> MEIVYKPLDIRNEEQFASIKKLIDADLSEPYSIYVYRYFLNQWPELTYIAVDNKSGTPNIPIGCIVCKMDPHRNVRLRGYIGMLAVESTYRGHGIAKKLVEIAIDKMQREHCDEIMLETEVENSAALNLYEGMGFIRMKRMFRYYLNEGDAFKLILPLT;> GPMEVDSILGSLSITDDFDQLVDVTSLFDELCSKLKPEAIVKDPRFDLFEGTHSLEVNNSKLDSSLIELTAEEIEFDVNVAYDPPLASVAAIADRLLRCVISWLNDYQTLPTTVLSCRYTESLLSSLVKGTTAGSSWCTGNILYDKVLGSCILGVCYLTKFVQKLLSAGIVFEEEDLNFNNMGFNTFDNLPGQDVVINSLTESLQILEAYSDDSLHLTMLKHILKIIICLVHLEDHLTDYSTKTSHLDELIENANSVNGIFPQLQLSPPKGAFSTYIQKHRSNQFPPRKITKLPTDYSGFITLANDVKTILLVDKAESALETYQFAKFFNKLEQRHVIARILFPLFFIRDDRTVLGKFSYTQFYLLHVKEFSAQTPSEFESSIGNELIQESSNMLLEWYQNCSQNTCRYRQGFNRQLILWDSLQAQFESVNSQVYCSWTYFMKLSSMIEFSLKGFDLDIYKPFEAYSMFWYVYYLSHHLETFLKDSQNDIESNINAIHSMNKKLKKLKAGEKKDQLRLKYRFAMDNEMEQLQATKQFLNYLLKEINITKSLCLIEVFQFAILKSFGLIDNKNSTPSKFSNERLIHNLRFKPFNSIGVPELPEYEVFQQTLKDFVIEEKGAAFDIKLERATNFIETEVRNVVSSIDEIMQGIKGGDNNGVLVTGTRLVQELSLEYYCKLKHTSKALSVNSKVIVNTLKKNIKNKDSHEYKVELVHTTEGWNYFPIQTLRIKQDRYK;> MDILKLSDFIGNTLIVSLTEDRILVGSLVAVDAQMNLLLDHVEERMGSSSRMMGLVSVPRRSVKTIMIDKPVLQELT;> MLRFVGSRRR

The transfer of an acetyl group from acetyl-coenzyme A to the free α-amino group on the N-terminus of substrate proteins is catalyzed by N-terminal acetyltransferases (NATs), and is considered to be irreversible, as no Nt-deacetylase has been identified so far. NatC acetylates protein N-termini starting with methionine, followed by a hydrophobic or amphipathic amino acid, with amino acids at positions 3 and 4 also contributing to NatC recognition. NatC forms a heterotrimeric complex, containing the catalytic subunit Naa30, the small auxiliary subunit Naa38 and the large auxiliary subunit Naa35. The large auxiliary subunit Naa35 acts as the central assembly hub of the NatC complex, forming extensive interactions with Naa30 and Naa38.

To obtain insights into the substrate recognition mode and the marked difference of NatC catalytic efficiencies toward the two peptides, crystal structures of NatC in complex with CoA, and either yArl3 or Gag peptide were determined to a maximal resolution of 2.99 and 2.75 Å, respectively. The electron density of the peptide ligands was sufficient to model the first four and six amino acids of the yArl3 and Gag peptide, respectively. At peptide position 3, Gag-Arg3 forms a hydrogen bond with the protein backbone and a cation–π interaction with Naa30-Tyr144. In addition, Naa30-Glu29 interacts with the Gag peptide backbone. Only in the Gag peptide, the fourth peptide residue, Phe4, deeply inserts into a second hydrophobic surface generated by Naa30 and Naa35, the “extended pocket”. In particular, binding of the Gag peptide induced a marked constriction of the central tunnel in NatC. Binding of Gag induces a flipping of Leu27, allowing recognition of the N-terminal methionine, which is sandwiched between Leu27 and Tyr145 of Naa30. In contrast to the yArl3 peptide, binding of the viral Gag peptide induced a large conformational rearrangement of the β6–β7 loop in Naa30. Naa30-Asn147 forms a hydrogen bond with Naa35-Gln106 in the apo and CoA/yArl3-bound NatC structures, but traversed a distance of 8.8 Å in the Gag-bound structure to form an intramolecular hydrogen bond with Naa30-Glu120. Moreover, Naa30-Leu146 moved ~5 Å toward Gag-Phe4, which complements the extended peptide pocket.Once inside the cell the terminal glycine is cleaved by a dipeptidase (PepA) to release Cys-3M3SH (2), which is metabolised by a C-S β-lyase liberating volatile 3M3SH (3), which diffuses or is exported out of the cell (4). While the PatB enzymes are poorly characterised and the genes are not associated with amino acid metabolism gene clusters or operons, the orthologues from B. subtilis (PatB) and Escherichia coli (MalY) are known to have cystathionine β-lyase activity, suggesting that these enzymes might also be capable of Cys-3M3SH cleavage. ShPatB and BsPatB are homodimeric with each subunit containing a PLP moiety covalently bound to a conserved lysine residue in the catalytic site (Lys246 and Lys234 in ShPatB and BsPatB, respectively) in what is termed the internal aldimine state. In the course of a typical PLP-DE catalysed reaction, upon substrate binding, the ε-amino group of the amino acid substrate displaces the lysine residue from the PLP to form an external aldimine.

The PatB enzymes from non-axillary microbes B. subtilis (BsPatB) and Streptococcus anginosus (SaPatB) did not discriminate between the two ligands, while the enzymes from Corynebacterium jeikeium (CjAecD) and E. coli MalY (EcMalY) had higher activities against cystathionine, similar to the MetC enzymes included (ShMetC and SeMetC), which have little or no activity against Cys-3M3SH. In contrast to ShPatB, the BsPatB binding cavity is more solvent exposed and composed of charged residues, thus enabling the binding of polar substrates like cystathionine and the hydroxyl group of the 3M3SH moiety of Cys-3M3SH.

>MNFDKREERLGTQSVKWDKTGELFGVTDALPMWVADMDFRAPEAITEALKERLDHGIFGYTTPDQKTKDAVCGWMQNRHGWKVNPESITFSPGVVTALSMAVQAFTEPGDQVVVQPPVYTPFYHMVEKNGRHILHNPLLEKDGAYAIDFEDLETKLSDPSVTLFILCNPHNPSGRSWSREDLLKLGELCLEHGVTVVSDEIHSDLMLYGHKHTPFASLSDDFADISVTCAAPSKTFNIAGLQASAIIIPDRLKRAKFSASLQRNGLGGLNAFAVTAIEAAYSKGGPWLDELITYIEKNMNEAEAFLSTELPKVKMMKPDASYLIWLDFSAYGLSDAELQQRMLKKGKVILEPGTKYGPGGEGFMRLNAGCSLATLQDGLRRIKAALS[4x]>MSRETNFNGTKRKRSDVAEKVAQRWKSVRYSAEMENMAPVNSNNDSDDCVIVSESKIIDLTNQEQDLSERIETNDTAKGAVFKLMKSDFYEREDFMGEVEDMITLKDIFGTETLKRSILFSFQYELDFLLRQFHQNVENITIVGQKGTIMPIEARAMDATLAVILKKVKLIEITMPPFASHHTKLIINFYDNGECKIFLPSNNFTSMETNLPQQVCWCSPLLKIGKEGLPVPFKRSLIEYLNSYHLKDIDELITKSVEEVNFAPLSELEFVYSTPSKFQSSGLLSFYNKLEKLSAGTSASDTAKHYLCQT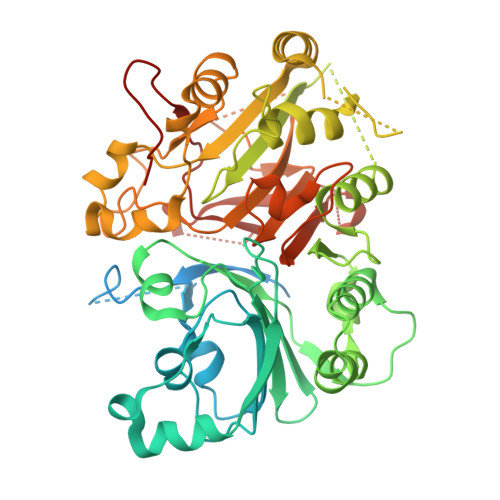SSIGTSLSRARDENLWTHLMIPLFTGIMSPPAKDTAGRKKAEILPTNSLINEYSQRKIKPYIIFPTEQEFVTSPLKWSSSGWFHFQYLQKKSYYEMLRNKFKVFYKQDPAMVTRRRGTTPAHSKFYMHCATNSAGPCDASQVFKELEWCLYTSANLSQTAWGTVSRKPRNYEAGVLYHSRRLANTRKVTCRTFTRDRRGCAGNPTHVAVPFTLPVIPYDLAEDECFCLARHEND[4x]The sialic acid transporter of P. mirabilis (SiaT) is a secondary active transporter of the SSS family, which use the Na+ electrochemical gradients as the driving force for the uptake of extracellular substrates. The uropathogen, Proteus mirabilis, catabolises host-derived sialic acids as a source of energy; the genes required for the transport and degradation of sialic acids are encoded within the nan operon. SiaT comprises 13 transmembrane helices (Tm0 and Tm1-Tm12) with the N- and C-termini facing the periplasmic and cytoplasmic spaces, respectively. Homologues of SiaT are found in a wide range of pathogenic bacteria including Streptococcus pneumoniae, S. enterica, Staphylococcus aureus and C. difficile.

Here we report the high-resolution (1.95 Å) substrate-bound outward-open structure and a functional and biophysical characterisation of SiaT. The structure is in complex with the sialic acid N-acetylneuraminic acid (Neu5Ac) and two Na+ ions. The sialic acid binding site is near the centre of the protein, lined by residues from four helices (Tm1-Tm3 and Tm6). The electron density in this site corresponds to Neu5Ac in its β-anomeric form as seen in the Haemophilus influenzae periplasmic binding protein (SiaP) of the sialic acid TRAP system. Tm1 and Tm6 adopt a distorted helical structure within the membrane bilayer at the point of contact with the substrate, which has implications for how binding drives the alternating-access mechanism. The negatively charged carboxylate group of Neu5Ac forms hydrogen bonds to the hydroxyl and amine groups of Ser60 and Thr63 and a salt bridge with the guanidinium of Arg135 (Tm3). One Na+ binds to the conserved Na2 site, whereas the second Na+ binds a new position that we term Na3. One ion occupies the conserved Na2 site, which is located between Tm1 and Tm8 at a prominent kink in Tm119. Na3 is 6.5 Å from Na2, towards the cytoplasm, and ~14 Å from the substrate binding site. At this position, the Na+ is coordinated by the main-chain carbonyl group of Ser342 (Tm8), the hydroxyl groups of Ser345 and Ser346 (Tm8), and by the carboxyl group of Asp182 (Tm5).

> MQLHDFGFINYAVLFGYLAAMLLVGVYFSKRQKTADDYFRGGGRVPGWAAGVSVFATTLSSITFMSIPAKAYTSDWTFIIGQYLAIAILPLVFYFYIPFFRKLKITSAYEYLEARFDVRSRLFASLSFMLFHIGRVAIITYLTVLALRPFMGIDPVVLIVLISLLCIIYTWMGGIEGVIWTDVIQGLLLSGGAVLIFIMICFKVDGGISEIFTTTAQADKFFPTTQWRWSWTDSTIPVLMIGFLFANIQQFTASQDVVQRYIVTDSIKETKRTLITNAKLVAIIPIFFFAIGSALFVYYQQNPSLLPAGFNTGGILPLFIVTEMPIGIAGLIIAAIFAAAQSSISSSLNSISSCFNSDIYTRLSKSSPSPEQKMKVAKLVIIVAGIFSSLAAIWLVLSDEAEIWDAFNSLIGLMGGPMTGLFMLGIFVKRANAGSAVVGIIVSIIAVLAARYGSDLNFFFYGVIGSMSVVIAGTITAPLFAPAKQLSLDDSETSEN> MADVKLHGSWVSPFNYRVIWALKLKGVEFEHIVEDLTNKSELLLKYNPVYKKIPVLVHGGKPIAESLVILEYIEETWPENPLLPTDPYERAMARFWIQYGATKTAAFGALFRASGEELEKAAKEVVEVLRVLEEQGLGDKKFFGGDSINLVDISFGLFTCWLEAIEEAAGVKVLEPSTLPRLHAWAQNFIEVPLIKENIPDYDKLLLHMKGVREKMMNK

Glutathione transferases (GSTs) constitute a widespread superfamily of enzymes notably involved in xenobiotic detoxification and/or in specialized metabolism. PtGSTU19 and 20, two paralogs sharing more than 91% sequence identity (95% of sequence similarity), would have diverged from a common ancestor of P. trichocarpa and P. yatungensis species. These enzymes display the distinctive glutathione (GSH)-conjugation and peroxidase activities against model substrates. PtGSTU19 and U20 have the same secondary structures as the known GSTU structures and show the canonical cytosolic GST fold.

The crystal structures of PtGSTU19 and 20 were solved in their apo form (U19 APO and U20 APO ) and in complex with GSH (U19 GSH and U20 GSH ). In PtGSTU20APO, no signal was found in the electronic density map corresponding to the region between β2 and β3, which includes helix α2 and its upstream and downstream loops (residues Glu34 to Lys51). In contrast, this region is well defined in the final electron density map of PtGSTU20GSH and PtGSTU20GSPAP and adopts the same conformation as observed in known GSTU structures including PtGSTU19APO/GSH. This region contains the invariant Lys39 that stabilizes the C-terminal carboxylate group of glutathione. PtGSTU20 has a valine residue at the beginning of the β2 to β3 region and not a glutamic acid as the other known GSTU crystal structures. Indeed, this latter residue participates in the stabilization of the region between β2 and β3 even in the absence of glutathione (see earlier). When a significant structural change is observed, α2 helix most often undergoes the most prominent rearrangement, as in the case of PtGSTU20. In PtGSTU19 and 20, glutathione binding induces two distinct stabilizations, β2 to β3 region for PtGSTU20 and α6 helix for PtGSTU19. In U20APO/GSH/GS-PAP, this tryptophan residue is buried (accessible surface area (ASA) of 4 Å2), making the H-site quite deep. A cysteine residue replaces Tyr160 in PtGSTU20 (Cys160) and only the first conformation is present whatever the form (U20APO/GSH/GSP).~{S}-[2-[3-[[(2~{R})-4-[[[(2~{R},3~{S},4~{R},5~{R})-5-(6-aminopurin-9-yl)-4-oxidanyl-3-phosphonooxy-oxolan-2-yl]methoxy-oxidanyl-phosphoryl]oxy-oxidanyl-phosphoryl]oxy-3,3-dimethyl-2-oxidanyl-butanoyl]amino]propanoylamino]ethyl] 3-oxidanylideneicosanethioate | C41 H72 N7 O18 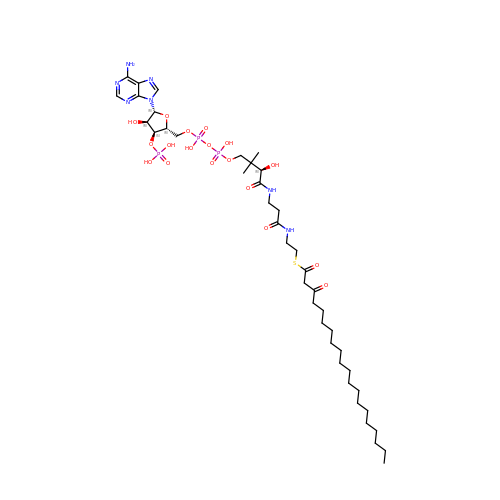P3 S | FYBVHNZJDVUVLJ-IBYUJNRCSA-N> MLDAFSKVITSADGKAAYVG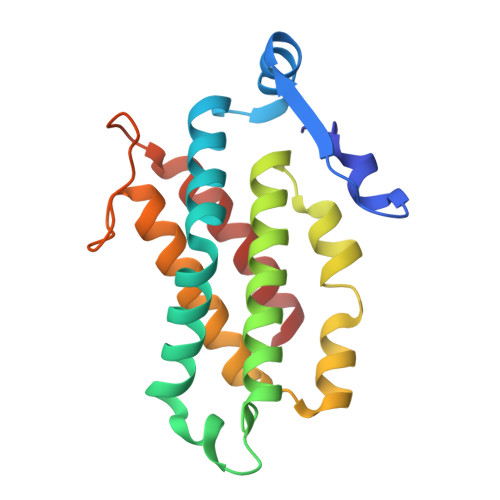GADLQALKKFVSEGNKRMDSVNAIVSNASCIVSDSVSGMVCENPSLIAPNGGVYTNRKMAACLRDAEIILRYVSYSLLSGDSSVLEDRCLNGLKETYASLGVPAAGNARTISIMKATVIGFITNNSQQKKLSTPAGDCSALASEVGGYFDKVSSALA>[2x]ETGSSRFQRVPQSQSVVENESVKFECESTDSYSELHYDWLHNGHRIAYDKRVHQIGSNLHIEAVRRTEDVGNYVCIATNLASGAREASPPAKLSVIYLESASVQLLGSNRNELLLKCHVEGASGDLEPLEIEWYRNSEKLSTWKNVQLDQHRLIIRQPGS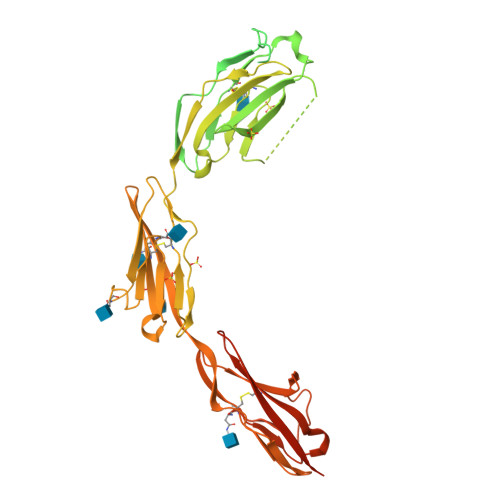EDDGLYRCTASNAAGRVMSKQGYVYQSSVKCLPRLPRRKNEKMMESWDKQTFLCRGKRGGAAGLEALPAAPEDLRIVQGPIGQSIIKEGEPTALTCLYELPDELKNQRIQLRWRKDGKLLRQVELGGSAPIPGHSFDSGKDALLREDARLVLHKQNGTLSFASIIASDAGQYQCQLQLEAHAPINSSPGILEVIEQLKFVPQPTSKNLELDAVVAKVHCKAQGTPTPQVQWVRDGENTTLPDHVEVDANGTLIFRNVNSEHRGNYTCLATNSQGQINATVAINVVVTPKFSVPPVGPIETSEQGTVVMHCQAIGDPKPTIQWDKDLKYLSENNTDRERFRFLENGTLEIRNVQVEDEGSYGCTIGNSAGLKREDVQLVVKTTGDGFAPEESGGDGFLVTRGTKHHHHHH>[2x]HHNKVRTCWNEGRPALAGWLQLPGTLHAEALARLDYDAVVIDMQASPIDFGQVAPMLIA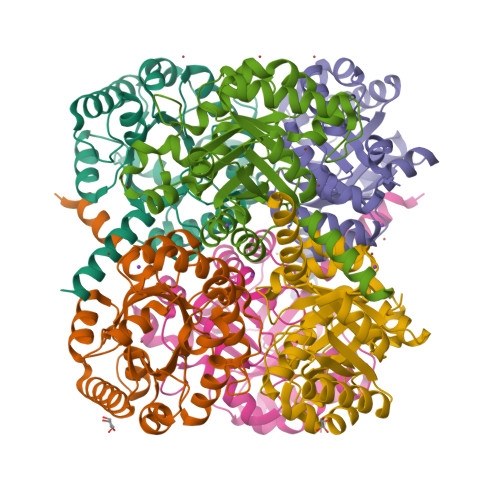IELGGAEPFVRTQVNDPSDIMKLLDAGAYGIIAPMVNTRAEAQTLASALHYSPRGLRSFGPRRPSLRYGSGYLAQASETVVGLAMIETREALANIDEILSVDGIDGVFIGPTDLALDLGHAPLVDTEEAEVVSAIAHVRERAHAAGKRVGIFCGSGGFARVKLAEGFDFVTAAPDLAMLSAAARQVIADARAL> MKITKRKWGEHHPPLYFYRDEDSGRLLAQNDRKQDYTDTLFNDIAQDTFERSLRNRLLKTPEKGDKRFYSNEIVKLVEKLCQGADVAEIMKSMERNEKLRPKNEKEIKNLKKQLDGTLSEYGKRYTAPEGAMTLNDALFYLVEGNPLKQAMAKAELGKIREALIKEKENRINRVRYSIKNNKIPLRIQEDGGITPNNDRAAWLLGLMKPADPAKGITDCYPLLGELEEVFDFDKLSKTLHEKISRCQGRPRSIAMAVDEALKQYLRELWEKSPSRQQDLKYYFQAVQEYFKDNFPIRTKRMGARLRQELLKDKTSLSRLLEPKHMANAVRRRLINQSTQMHILYGKLYAYCCGEDGRLLVNSETLQRIQVHEAVKKQAMTAVLWSISRLRYFYQFEDGDILSNKNPIKDFRDKFLRDTNKYTHEDVEACKEKLQDFFPLKELQEKIKEDAKGLQETDNKQADTTDFKAIGHIVRDDRKLCNQLLAECVSCIGELRHHIFHYKNVTLIQALKRIADKVKPEDLSVLRAIYLLDRRNLKKAFAKRISSMNLPLYYREDLLSRIFKKEGTAFFLYSAKIQMTPSFQRVYERGKNLRREFECERMKAEASNGQNGQDGDRLKWFRQLAAGDSADTHFNWAVEAYAESAADVENNVEFDTDVDAQRALRNLLLLIYRHHFLPEVQKDETLVTGKIHKVLERNRQLSEGQGPNQGKAHGYSVIEELYHEGMPLSDLMKQLQRRISETERESRELAQEKTDYAQRFILDIFAEAFNDFLEAHYGEEYLEIMSPRKDAEAAKKWVKESKTVDLKTSIDEKEPEGHLLVLYPVLRLLDERELGELQQQMIRYRTSLASWQGESNFSEEIRIAGQIEELTELVKLTEPEPQFAEEVWGKRAKEAFEDFIEGNMKNYEAFYLQSDNNTPVYRRNMSRLLRSGLMGVYQKVLASHKQALKRDYLLWSEKHWNVKDENGADISSAEQAQCLLQRLHRKYAESPSRFTEEDCKLYEKVLRRLEDYNQAVKNLSFSSLYEICVLNLEILSRWVGFVQDWERDMYFLLLAWVRQGKLDGIKEEDVRDIFSEGNIIRNLVDTLKGENMNAFESVYFPENKGSKYL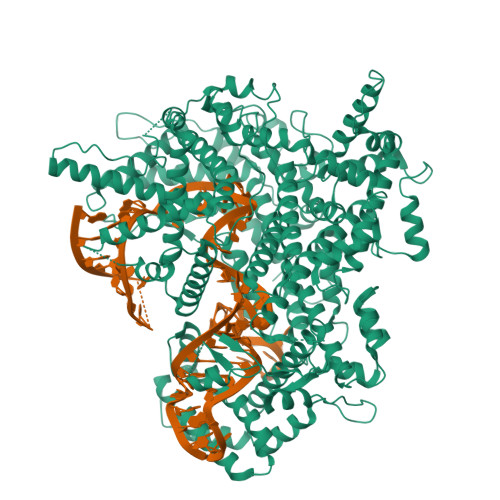GVRNDVAHLDLMRKNGWRLEAGKTCSVMEDYINRLRFLLSYDQKRMNAVTKTLQQIFDRHKVKIRFTVEKGGMLKIEDVTADKIVHLKGSRLSGIEIPSHGERFIDTLKALMVYPRG(3~{S})-3-azanylazepan-2-one | C6 H12 N2 O | 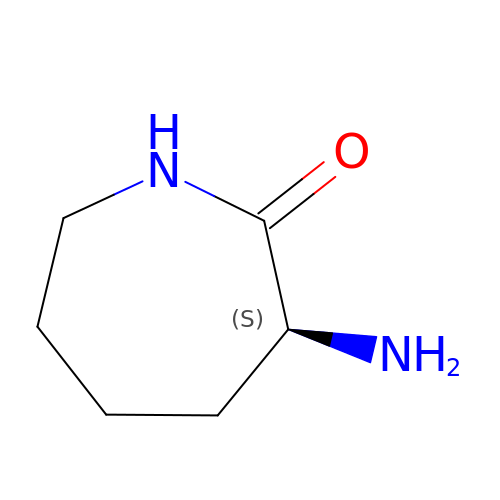BOWUOGIPSRVRSJ-YFKPBYRVSA-N> GAMASGKVVKFSYMWTINNFSFCREEMGEVIKSSTFSSGANDKLK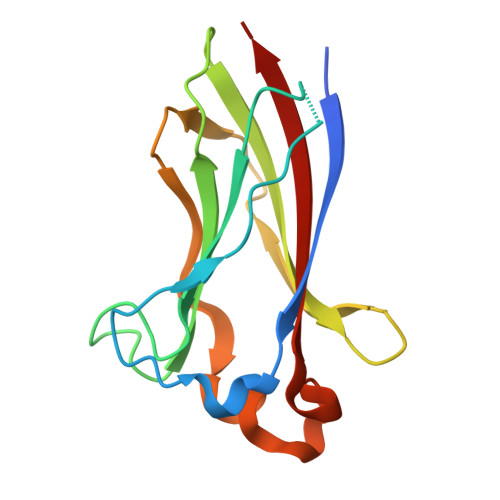WCLRVNPKGLDEESKDYLSLYLLLVSCPKSEVRAKFKFSILNAKGEETKAMESQRAYRFVQGKDWGFKKFIRRNFLLDEANGLLPDDKLTLFCEVSVVQD[1-(3-chlorophenyl)-1H-pyrazol-4-yl]boronic 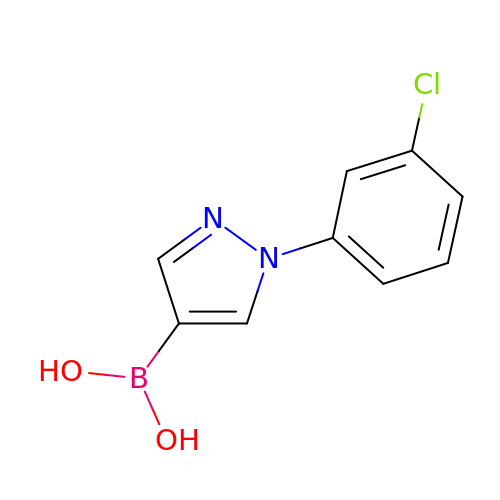acid | C9 H8 B Cl N2 O2 | QQIIJLJSZUIAKB-UHFFFAOYSA-N3,3',3'',3'''-[(1R,2S,3S,4S,7S,8S,11S,12S,13S,16S,19S)-3,8,13,17-tetrakis(carboxylatomethyl)-8,13-dimethyl-1,2,3,4,7,8,11,12,13,16,19,20,22,24-tetradecahydroporphyrin-2,7,12,18-tetrayl]tetrapropanoate | C42 H52 N4 O16 | 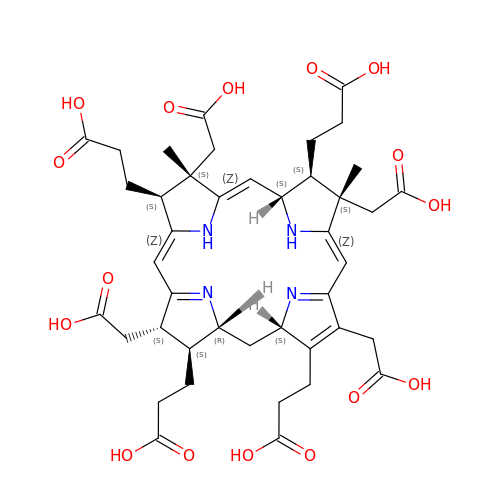PTDGOSZHGZMQAZ-IIRIWOCESA-N1-{2-[(2S)-2-{[(3-chloro-2-fluorophenyl)methyl]carbamoyl}pyrrolidin-1-yl]-2-oxoethyl}-1H-indazole-3-carboxamide | C22 H21 Cl F N5 O3 | 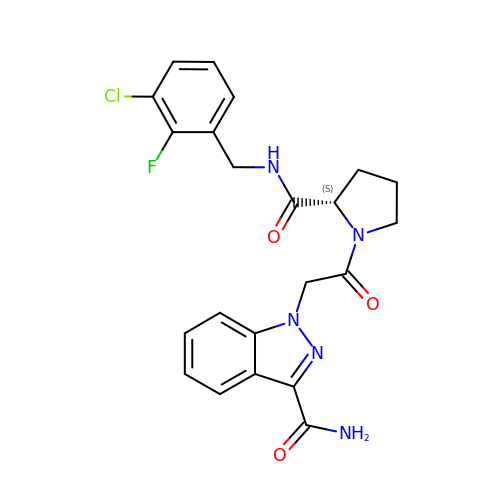CNXBYALMVOPTMF-KRWDZBQOSA-N>[2x]MSLRIGVIGTGAIGKEHINRITNKLSGAEIVAVTDVNQEAAQKVVEQYQLNATVYPNDDSLLADENVDAVLVTSWGPAHESSVLKAIKAQKYVFCEVPLATTAEGCMRIVEEEIKVGKRLVQVGFMRRYDSGYVQLKEALDNHVIGEPLMIHCAHRNPTVGDNYTTDMAVVDTLVHEIDVLHWLVNDDYESVQVIYPKKSKN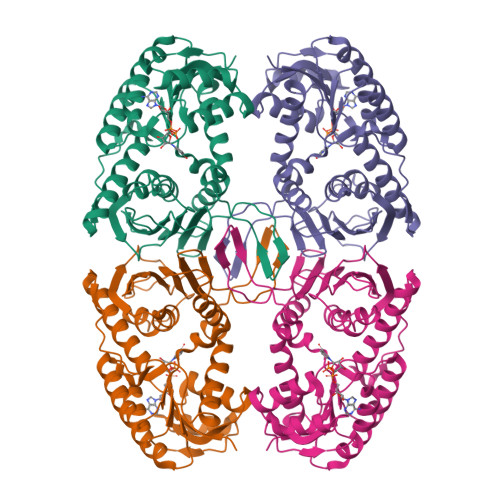ALPHLKDPQIVVIETKGGIVINAEIYVNCKYGYDIQCEIVGEDGIIKLPEPSSISLRKEGRFSTDILMDWQRRFVAAYDVEIQDFIDSIQKKGEVSGPTAWDGYIAAVTTDACVKAQESGQKEKVELKEKPEFYQSFTTVQN> AQLVIMTIALSLATFMQVLDSTIANVAIPTIAGNLGSSLSQGTWVITSFGVANAISIPLTGWLAKRVGEVKLFLWSTIAFAIASWACGVSSSLNMLIFFRVIQGIVAGPLIPLSQSLLLNNYPPAKRSIALALWSMTVIVAPICGPILGGYISDNYHWGWIFFINVPIGVAVVLMTLQTLRGRETRTERRRIDAVGLALLVIGIGSLQIMLDRGKELDWFSSQEIIILTVVAVVAICFLIVWELTDDNPIVDLSLFKSRNFTIGCLCISLAYMLYFGAIVLLPQLLQEVYGYTATWAGLASAPVG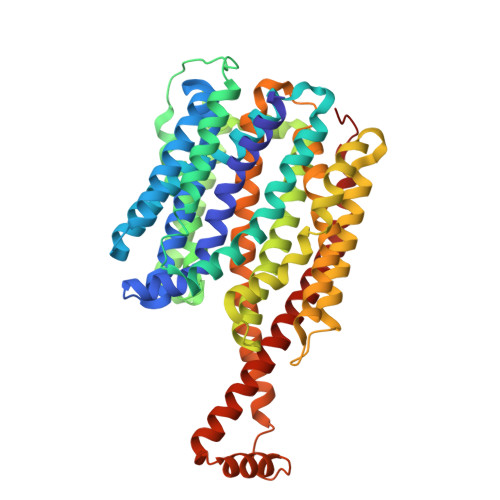IIPVILSPIIGRFAHKLDMRRLVTFSFIMYAVCFYWRAYTFEPGMDFGASAWPQFIQGFAVACFFMPLTTITLSGLPPERLAAASSLSNFTRTLAGSIGTSITTTMWTNRESMHHAQLTESVNPFNPNAQAMYSQLEGLGMTQQQASGWIAQQITNQGLIISANEIFWMSAGIFLVLLGLVWFAKPPFG6-({(1R)-1-[2-methyl-3-(trifluoromethyl)phenyl]ethyl}amino)-8-(oxan-4-yl)-1,3,4,8-tetrahydropyrido[3,4-c][1,6]naphthyridin-9(2H)-one 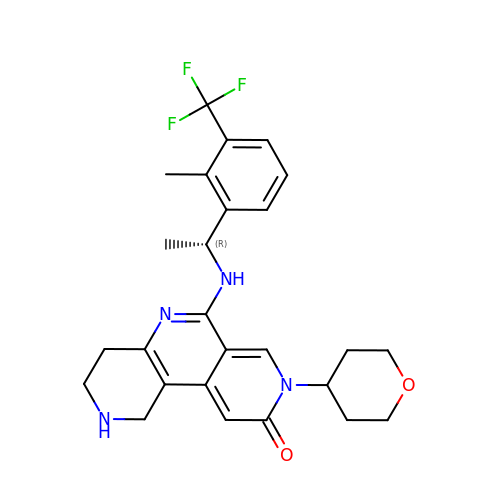| C26 H29 F3 N4 O2 | ALSMRGTYWDRDTI-MRXNPFEDSA-N>HHHHHSDIRAVVYGVGAMNSIVAGMLLDKGVQIVGAIARSPQKVGQDLGDLLGLGRQLGVAVSDDAAEVLEQTHPDIAVIAVNSYLTDAVEQLRICAEHGVNAVTLSEEMLYPWETSPELSAELDALAKSTGATLTGTGYQDTFWVNMIALLMGTAHRIDTVRGKASWNVDDFGPELATAQQVGRTVAEFDEWVRGAQRPPTFGRNVLDALVADTGLTVKSITTATRPDIASAAMRSEALGIDLAPGDVIGFTDIDRIETEEGPVFEFEMSGRVYGPGEGDINEWTIEGEPNLFLSNGTVPTQTTTCTQMVNRIPDVIAAPPGIVTVDRLPRL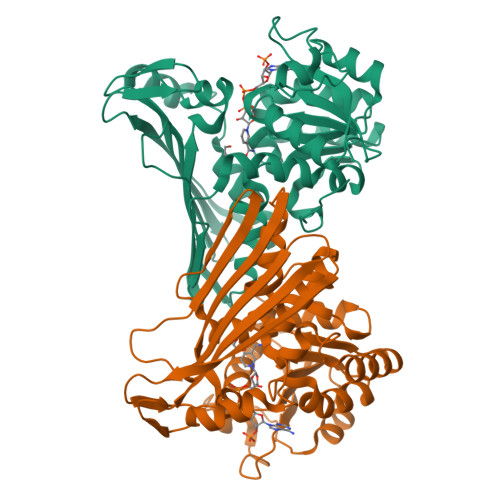RYRPQF[4x]>ASSSSSMALGRIGEVKRVTKETNVSVKINLDGTGVADSSSGIPFLDHMLDQLASHGLFDVHVRATGDVHIDDHHTNEDIALAIGTALLKALGERKGINRFGDFTAPLDEALIHVSLDLSGRPYLGYNLEIPTQRVGTYDTQLVEHFFQSLVNTSGMTLHIRQLAGENSHHIIEATFKAFARALRQATETDPRRGGTIPSSK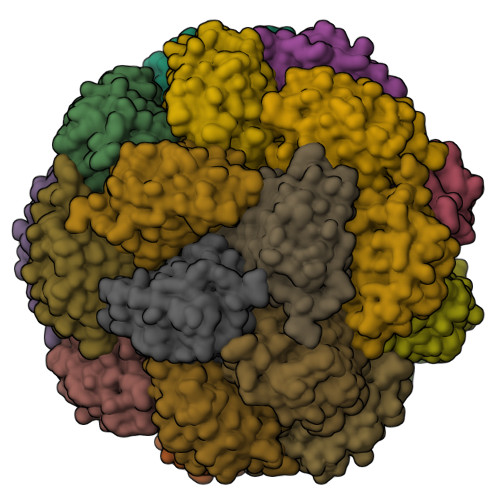GVLSRS[16x]>GSLDGPYQSTSFKPPSDYWILLNPTNQQVVLEGTNKTDIWVALLLVEPNVTNQSRQYTLFGETKQITVENNTNKWKFFEMFRSSVSAEFQHKRTLTSDTKLAGFLKHYNSVWTFHGETPHATTDYSSTSNLSEVETTIHVEFYIIPRSQESKCVEYINTGL[2x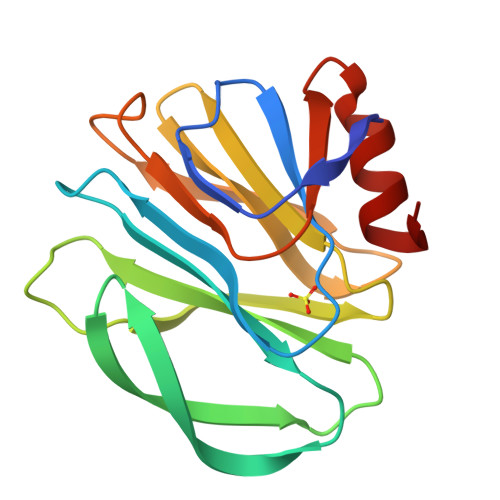]> MAAKTIPFVASTALGERLFAGVQKVLAAAKAPVSLVQTDAKFAPADAKYLLAEPLSAAATGELANKYGLSSKVTSGAASQFYPNSIYPSLNVEVVQNLYALSNPAFSSLSATTTKAVTVKDESAIKLAELQKETERNISSFFRDEANKSVQATLRLACDKAIKTKADKKTVMVVTKPHGDAFDDLLAQVTKSESDGRADELRNSSVSVEPTLVGNAWPKLVMFPE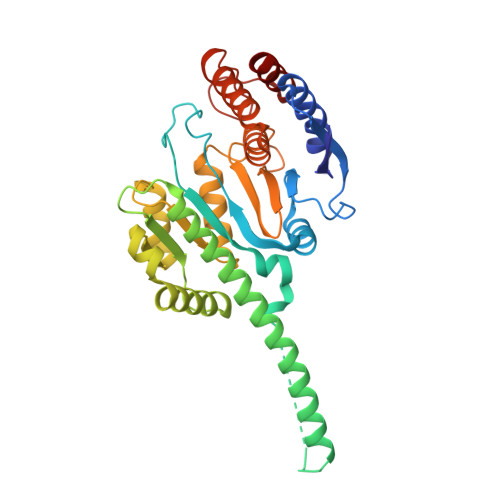GVNVVVCGPNASGDQVAQLFVGIAGGTGMVAQQLVGDAVVFTSANAEDNENPTGALLAASNLLTALGHEAEAKKIAAAVAKAYTTDRILPKELPGGKADLEAFIDAVAKHASA>[2x]GPHMASARERENLQLKLEQIRHSLEDDLDLRSDPAVQ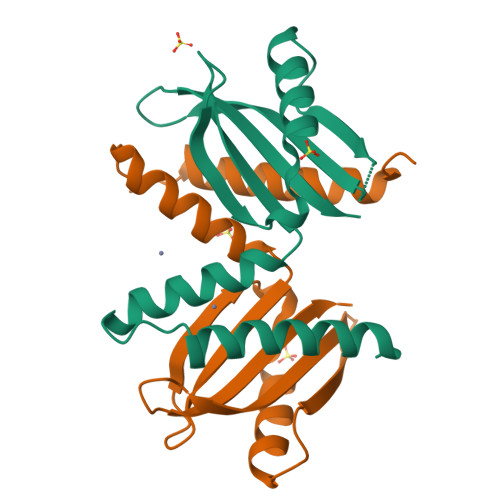AHALQDQLVAHSGLHLSILDSRSGQPLMSFGDQAAASVAANRALLARLQADARQPVFQSWSTGNDQRLLSIGASMRMKNGTPVQVLLSSERNADE>[2x]MESNEDVERLLCQKYPGL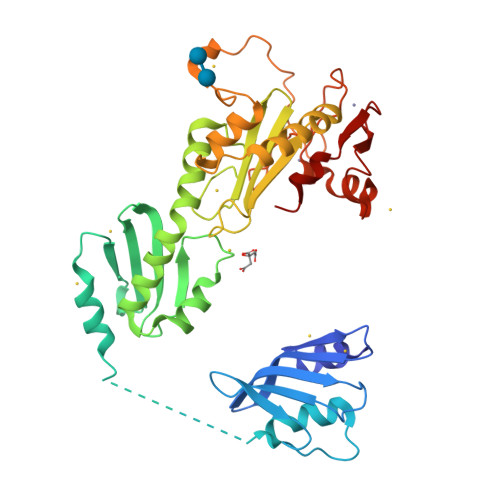AAELQPSGACIIRGVLGSEDTWRRLKLYLPHHPALHGFQLYVQESLEYKLYTSANLKLQDDWLLEDFLDHLPKILPAQKAPTVPKELCREGNIYYDILALYKSNEYCLQVDEACSMIRFSEFTDFEQHYLELKIPSLLLLDHSLPDCVSLGEMLTKSAGNLEEALNLFRKLLEDLRPFYDNFMDIDELCHVLQPSPISSKHKTRLFPLKDRVYLKLTIADPFACIASMSLKIIGPTEEVARLRHVLSDGLSNWDSEMNIHKNLLRMFDLCYFPMPDWSDGPKLDEEDNEELRCNICFAYRLDGGEVPLVSCDNAKCVLKCHAVCLEEWFKTLMDGKTFLEVSFGQCPFCKAKLSTSFAALLND>MNLPTAQEVQGLMARYIELV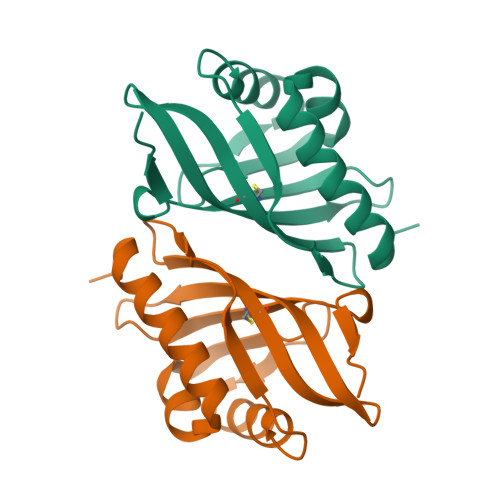DVGDIEAIVQMYADDATVENPFGQPPIHGREQIAAFYRQGLGGGKVRASLTGPVRASHNGSGAMPCRVEMVWNGQPSALDVIDVMRFDEHGRIQTMQAYWSEVNLSVREPQ[4x]5 is an essential electron transfer protein, which is ubiquitously found in living systems and involved in wide variety of biological processes. Tardigrades (also known as water bears), some of which are famous for desiccation resistance, have many proteins unique to them. 5 do not have a C‐terminal transmembrane helix, which anchors the proteins on microsomal or mitochondrial membranes; therefore, they are soluble proteins. 5, are distinguished from others by insertion of amino acid residues which we named tardigrade specific loop (TS loop).

The crystal structure was determined at a resolution of 1.4 Å by a single‐wavelength anomalous dispersion method using a heme iron atom (Fe‐SAD). The electron density map indicates that there are three different conformations of heme. 5 proteins is a presence of a TS loop between β3 and β4. Although the TS loop does not form any secondary structures, the residues on it form a hydrogen bond network with each other and a salt bridge between Asp36 and Arg45. The TS loop shows few interactions with surrounding residues outside the TS loop, implying that it can flexibly move independent of other parts of the protein. One interaction is a hydrogen bond formed by the carbonyl O atom of Ser42 and the side chain of Arg35. The second one is a guanidino group stacking between Arg45 and Arg92. 5, the surface surrounding the heme binding site and a cleft made by the TS loop are positively charged. 5 is thought to interact with proteins having negatively charged surfaces around their redox centers.

> HHHHHHSSENLYFQSLRKDKAEEQTFSWSEISQHTSANSLWVVVRDKTSPGSPLRVYDVTNFQKTHPGGHLILLKYAGTECSRAFAAVGHSKYAIKRMSQYRIGIAEADNVE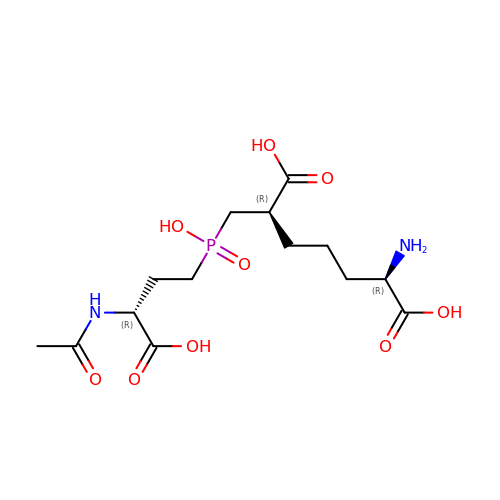(2R,6R)-2-{[(R)-[(3R)-3-(acetylamino)-3-carboxypropyl](hydroxy)phosphoryl]methyl}-6-aminoheptanedioic acid | C14 H25 N2 O9 P | AWMPEAXWUINOES-HBNTYKKESA-N>GSQKERLLDELTLEGVARYMQSERCRRVICLVGAGISTSAGIPDFRSPSTGLYDNLEKYHLPYPEAIFEISYFKKHPEPFFALAKELYPGQFKPTICHYFMRLLKDKGLLLRCYTQNIDTLERIAGLEQEDLVEAHGTFYTSHCVSASCRHEYPLSWMKEKIFSEVTPKCEDCQSLVKPDIVFFGESLPARFFSCMQSDFLKVDLLLVMGTSLQVQPFASLISKAPLSTPRLLINKEKAGGGGMDFDSKKAYRDVAWLGECDQGCLALAELLGWKKELEDLVRREHASI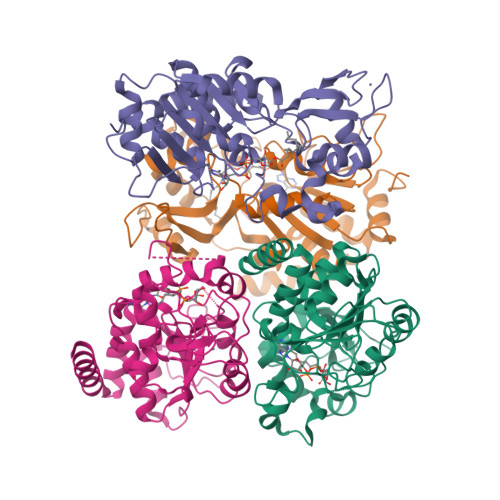DAQS[4x]> MVDQATLDKLEAGFKKLQEASDCKSLLKKHLTKDVFDSIKNKKTGMGATLLDVIQSGVENLDSGVGIYAPDAESYRTFGPLFDPIIDDYHGGFKLTDKHPPKQWGDINTLVGLDPAGQFIISTRVRCGRSLQGYPFNPCLTAEQYKEMEEKVSSTLSSMEDELK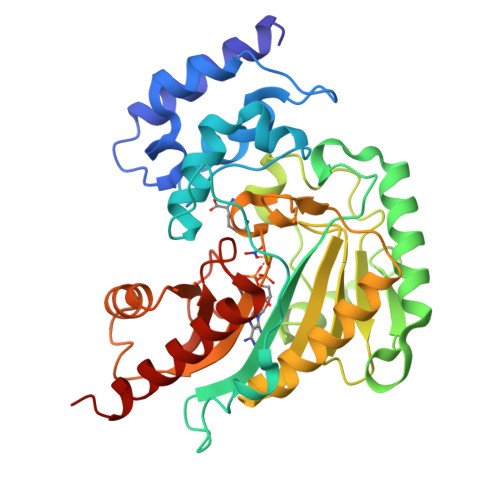GTYYPLTGMSKATQQQLIDDHFLFKEGDRFLQTANACRYWPTGRGIFHNDAKTFLVWVNEEDHLRIISMQKGGDLKTVYKRLVTAVDNIESKLPFSHDDRFGFLTFAPTNLGTTMRASVHIQLPKLAKDRKVLEDIASKFNLQVRGTRGEHTESEGGVYDISNKRRLGLTEYQAVREMQDGILEMIRMEKAAA> MISRVTEALSKVKGSMG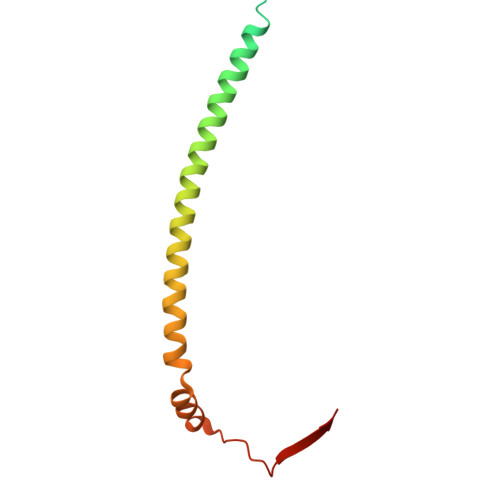SHERHALPGVIGDDLLRFGKLPLCLFICIILTAVTVVTTAHHTRLLTAQREQLVLERDALDIEWRNLILEENALGDHSRVERIATEKLQMQHVDPSQENIVVQK>[4x]MLPGKAVEIPAGDHLWKSASPAAPRPSGSTYMGGFKAPRLGRIRLAFIGVGGRGFSHLAQMCVMDGVEIVGICDLKEELTKRGVDRVLSRMGKSPLGYSGGDMEYLTMLKELKPDAVIIST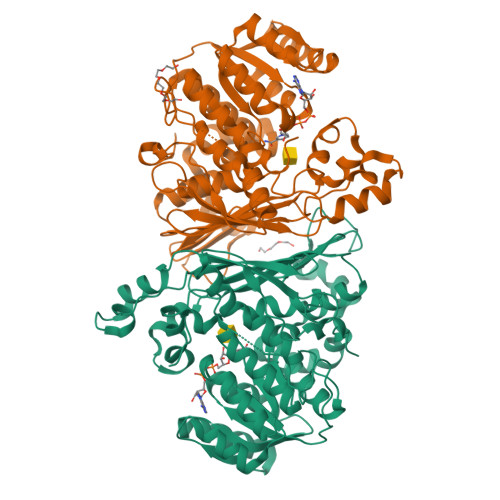DWSSHARIACDSMKHGAHAFVEVPLAVSLEELWSLVDTSEATRKHCMMMENVNYGRDELMFLNMVRQGVIGDLLHGEAAYIHCLVTQLGDTRGEGAWRPEYHTRINGNLYPTHGLGPVAQYMNLERGEDRFCRVAAFASPALGRNAYAKKHLPADHRWNNTPFICGDMNTAVVKTQLGRTILVQLDETSPRPYSRANLIQGTEGTLAGFPTRVAGEKLGNGNYHEWIEGREKLAAIYEKYDHPLWKRIGELATKMGGHGGMDFVMLSRIVECLRNGEPMDQNVYEGASWSSLLPLTARSIAQGGMPVEFPDFTRGDWKTTMPLAVVSLEHHHHHH>[2x]GPAM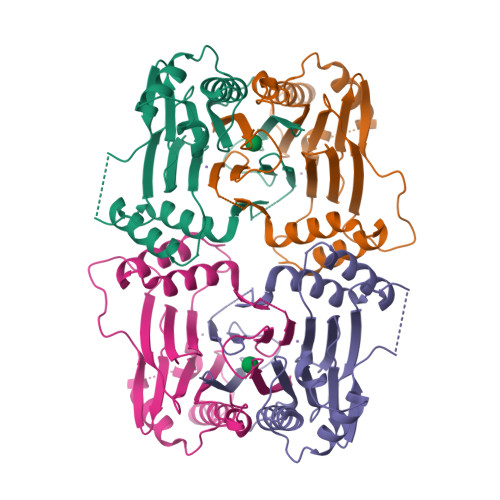SYRVSTGAAHAAKGGGLVSGDSYSMMELGARKYAAAISDGMGNGARAHFESNETIKLLEKILESGIDEKIAIKTINSILSLRTTDEIYSTLDLSIIDLQDASCKFLKVGSTPSFIKRGDQVMKVQASNLPIGIINEFDVEVVSEQLKAGDLLIMMSDGIFEGPKHVENHDLWMKRKMKGLKTNDPQEIADLLMEEVIRTRSGQIEDDMTVVVVRIDHNTPKWASIPVPAIFQNKQEIS> GVENAEKGVTENTDATADFVAQPVYLPENQTKVAFFYDRSSPIGAFAVKSGSLESGFAPFSNKACPNSVILTPGPQFDPAYDQLRPQRLTEIWGNGNEETSEVFPLKTKQDYSFCLFSPFVYYKCDLEVTLSPHTSGAHGLLVRWCPTGTPTKPTTQVLHEVSSLSEGRTPQVYSAGPGTSNQISFVVPYNSPLSVLPAVWYNGHKRFDNTGDLGIAPNSDFGTLFFAGTKPDIKFTVYLRYKNMRVFCPRPTVFFPWPTSGDKIDMTPRAGVLMLE;> DQNTEEMENLSDRVSQDTAGNTVTNTQSTVGRLVGYGTVHDGEHPASCADTASEKILAVERYYTFKVNDWTSTQKPFEYIRIPLPHVLSGEDGGVFGATLRRHYLVKTGWRVQVQCNASQFHAGSLLVFMAPEYPTLDVFAMDNRWSKDNLPNGTRTQTNRKGPFAMDHQNFWQWTLYPHQFLNLRTNTTVDLEVPYVNIAPTSSWTQHASWTLVIAVVAPLTYSTGASTSLDITASIQPVRPVFNGLRHEVLSRQ;> SPIPVTIREHAGTWYSTLPDSTVPIYGKTPVAPANYMVGEYKDFLEIAQIPTFIGNKVPNAVPYIEASNTAVKTQPLAVYQVTLSCSCLANTFLAALSRNFAQYRGSLVYTFVFTGTAMMKGKFLIAYTPPGAGKPTSRDQAMQATYAIWDLGLNSSYSFTVPFISPTHFRMVGTDQANITNVDGWVTVWQLTPLTYPPGCPTSAKILTMVSAGKDFSLKMPISPAPWSPQ;> GNSTSSDK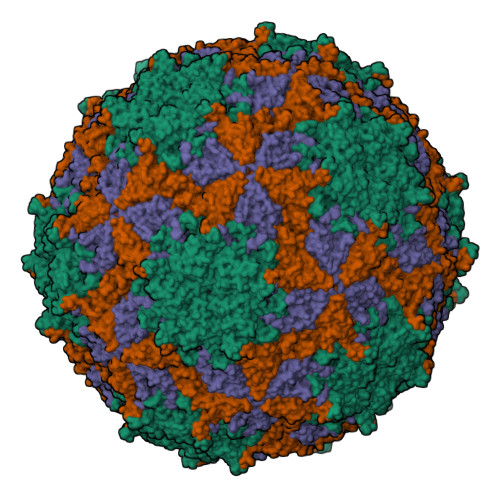NNSSSEGNEGVIINNFYSNQYQNSIDLSANATGSDPPKTYGQFSNLLSGAVNAFSNMLPLLA> MSNVQTSAEREIVDLSHLAFDCGMLGRLKTVSWTPVIAGDSFELDAVGAL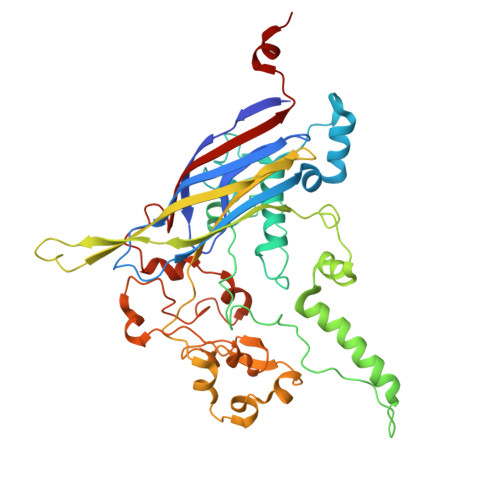RLSPLRRGLAIDSKVDFFTFYIPHRHVYGDQWIQFMRDGVNAQPLPSVTCNRYPDHAGYVGTIVPANNRIPKFLHQSYLNIYNNYFRAPWMPERTEANPSNLNEDDARYGFRCCHLKNIWSAPLPPETKLAEEMGIESNSIDIMGLQAAYAQLHTEQERTYFMQRYRDVISSFGGSTSYDADNRPLLVMHTDFWASGYDVDGTDQSSLGQFSGRVQQTFKHSVPRFFVPEHGVMMTLALIRFPPISPLEHHYLAGKSQLTYTDLAGDPALIGNLPPREISYRDLFRDGRSGIKIKVAESIWYRTHPDYVNFKYHDLHGFPFLDDAPGTSTGDNLQEAILVRHQDYDACFQSQQLLQWNKQARYNVSVYRHMPTVRDSIMTS> SENSLEIEELARFAVDEHNKKENALLEFVRVVKAKEQHQFHMSWTWTMYYLTLEAKDGGKKKL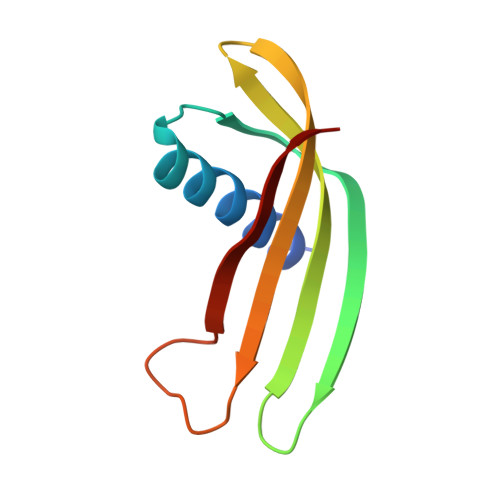YEAKVWVKHHPAYIADINFKELQEFKPV Retromer is a master regulator of cargo retrieval from endosomes, which is critical for many cellular processes including signaling, immunity, neuroprotection, and virus infection. The core of retromer is a trimer comprising vacuolar protein sorting (VPS) proteins VPS35, VPS26, and VPS29. Here, we elucidate the structural basis of membrane tubulation and coupled cargo recognition by metazoan and fungal retromer coats assembled with the non–Bin1/Amphiphysin/Rvs (BAR) sorting nexin SNX3 using cryo–electron tomography. The retromer core retains its arched, scaffolding structure but changes its mode of membrane recruitment when assembled with different SNX adaptors, allowing cargo recognition at subunit interfaces.

In fungi, the only known non–BAR-containing SNX adaptor is the SNX3 homolog, Grd19 (13, 19). Comparison of the assemblies demonstrated that metazoan and fungal coats are essentially identical, and hereafter, we describe metazoan retromer:SNX3 unless stated otherwise. Using local reconstruction and three-dimensional (3D) classification, we found that, for both metazoan and fungal retromer:SNX3 datasets, the arch is asymmetrical. One VPS35 monomer is more curved than the other, and the two monomers interact via an asymmetric VPS35:VPS35 dimerization interface. This asymmetry causes the arches to tilt by approximately 22° away from the perpendicular relative to the membrane. Arches were arranged in a pseudohelical lattice wound around membrane tubules. The fungal retromer:Grd19 lattice shows less regularity than either the metazoan retromer:SNX3 or the previously described fungal retromer:SNX-BAR lattice. Arches are assembled into linear chains via two homodimerization interfaces—the asymmetrical VPS35 dimer interface and the symmetrical VPS26 dimer interface. The core trimer arch—the conserved architectural element of the different retromer coats—forms a scaffold that can contribute directly or indirectly to membrane bending and which propagates curvature over larger areas of membrane by oligomerization.

>[2x]MSTPAPPEEQARLLEDALIAVRQQTAMMRKFLDTPGKLMDALKCCSTLVSELRTSSLSPKQYYELYMAVFDALRYLSAHLRENHPVNHLADLYELVQYAGNIIPRLYLMITVGTAYMSIDGAPVKELMKDMMDMSRGVQHPVRGLFLRYYLSGQARDYLPTGDSDGPEGNLQDSINFILTNFVEMNKLWVRLQHQGHSRERDLRTQERRELQLLVGSNIVRLSQLVDLPTYRDSILGPLLEQIVQCRDILAQEYLLEVITQVFPDEYHLHTLDQFLGAVSRLNPHVNVKAIVIGMMNRLSDYAERESQNEPEEDRAKLEEEALAKLLEKTKLGQNSELEPQNGDHPDTEVSSTTDSAQAPSTADSDTTAVNGEEEPVRKRRGIPVNVPLYDIFFDQVQHLVQAQHLPIQDTIALCCSLANLSLNIYPERLDYVDGILAYALAKVKEHANSADLHSQPAQQSLLSLLQSPLRRYVSIFTALSLPTYVSLFQAQTYPTRRAIAGEIVRTLLKNQTLISTPAHLENVLEILKVLIKEGSQPPAGYPGVVQPRARPLETDETMEEQGWLARLVHLIHSDDNDTQFRLLQMTRKAYAEGNERIRTTTPPLITAGLKLARRFKAREHYDDNWSSQSSSLFKFLHSAISTLYTRVNGPGVADLCLRLFCSCGQVADMTEFEEVAYEFFAQAFTVYEESISDSKAQFQAVCVIASALHRTRNFGRENYDTLITKCAQHASKLLRKPDQCRAVYLASHLWWATPIAARGETEDTELYRDGKRVLECLQRALRVADSCMETATSIELFVEILDRYVYYFDQRNESVTTKYLNGLIELIHSNLAGNQQDSASVEASRKHFIQTLEMIQSKEFEGIVVAPK;>[2x]SMAFLILVIGNLHIPDRALDIPPKFKKLLSPGKISQTLCLGNLTDRATYDYLRSISPDLKIVRGRMDVEATSLPLMQVVTHGSLRIGFLEGFTLVSEEPDVLLAEANKLDVDVLCWAGGSHRFECFEYMDKFFVNPGSATGAFTTDWLAEGEEVVPSFCLMDVQGISLTLYVYQLRKDENGTENVAVEKVTYTKPVEPTGAS> DFDFEGNLALFDKAAVFEEIDTYERRSGTRSRGIPNERPTRYRHDENILESEPIVYRRIIVPHNVSKEFCTDSGLVVPSISYELHKKLLSVAEKHGLTLERRLEMTGVCASQMALTLLGGPNRLNPKNVHQRPTVALLCGPHVKGAQGISCGRHLANHDVQVILFLPNFVKMLESITNELSLFSK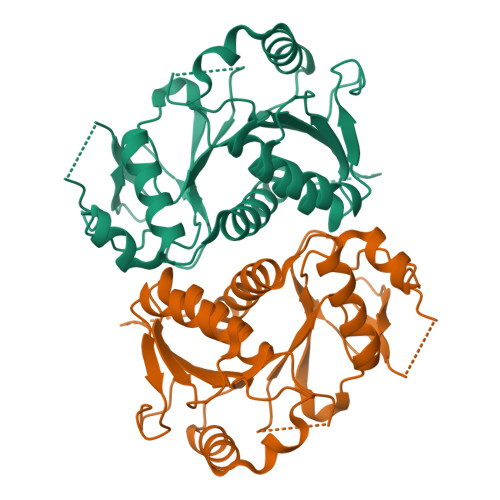TQGQQVSSLKDLPTSPVDLVINCLDCPENVFLRDQPWYKAAVAWANQNRAPVLSIDPPVHEVEQGIDAKWSLALGLPLPLGEHAGRIYLCDIGIPQQVFQEVGINYHSPFGCKFVIPLHSA> MSVHATDAKPPGPSPADQLLDGLNPQQRQAVVHEGSPLLIVAGAGSGKTAVLTRRIAYLMAARGVGVGQILAITFTNKAAAEMRERVVGLVGEKARYMWVSTFHSTCVRILRNQAALIEGLNSNFSIYDADDSRRLLQMVGRDLGLDIKRYSPRLLANAISNLKNELIDPHQALAGLTEDSDDLARAVASVYDEYQRRLRAANALDFDDLIGETVAVLQAFPQIAQYYRRRFRHVLVDEYQDTNHAQYVLVRELVGRDSN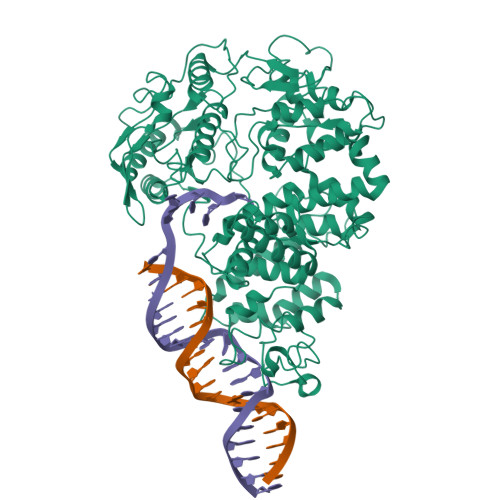DGIPPGELCVVGDADQSIYAFRGATIRNIEDFERDYPDTRTILLEQNYRSTQNILSAANSVIARNAGRREKRLWTDAGAGELIVGYVADNEHDEARFVAEEIDALAEGSEITYNDVAVFYRTNNSSRSLEEVLIRAGIPYKVVGGVRFYERKEIRDIVAYLRVLDNPGDAVSLRRILNTPRRGIGDRAEACVAVYAENTGVGFGDALVAAAQGKVPMLNTRAEKAIAGFVEMFDELRGRLDDDLGELVEAVLERTGYRRELEASTDPQELARLDNLNELVSVAHEFSTDRENAAALGPDDEDVPDTGVLADFLERVSLVADADEIPEHGAGVVTLMTLHTAKGLEFPVVFVTGWEDGMFPHMRALDNPTELSEERRLAYVGITRARQRLYVSRAIVRSSWGQPMLNPESRFLREIPQELIDWRRTAPKPSFSAPVSGAGRFGSARPSPTRSGASRRPLLVLQVGDRVTHDKYGLGRVEEVSGVGESAMSLIDFGSSGRVKLMHNHAPVTKL>[2x]ADTKEVLEAREAYFKSLGGSMKAMTGVAKAFDAEAAKVEAAKLEKILATDVAPLFPAGTSSTDLPGQTEAKAAIWANMDDFGAKGKAMHEAGGAVIAAANAGDGAAFGAALQK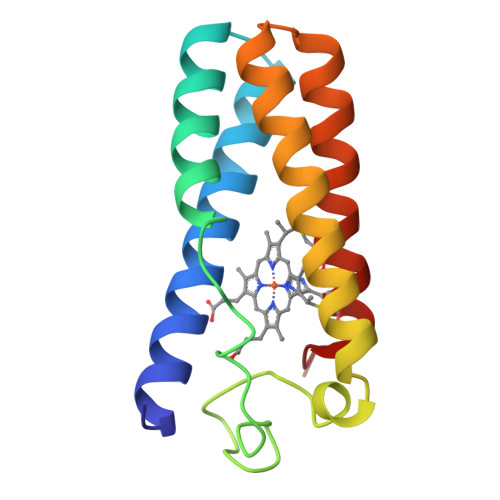LGGTCKACHDDYREED>[2x]GSHMMPQLQFKDAFWCRDFTAHTGYEVLLQRLLDGRKMCKDMEELLRQRAQAEERYGKELVQIARKAGGQTEINSLRASFDSLKQQMENVGSSHIQLALTL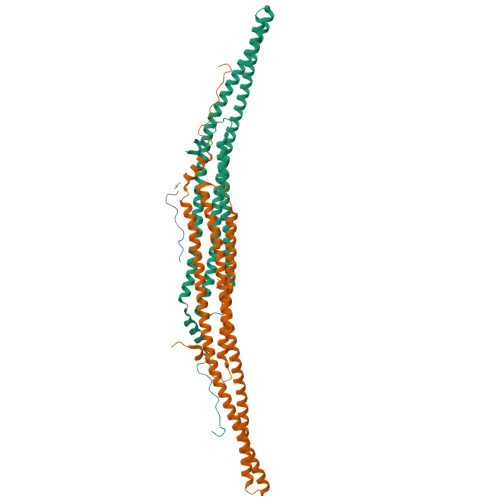REELRSLEEFRERQKEQRKKYEAVMDRVQKSKLSLYKKAMESKKTYEQKCRDADDAEQAFERISANGHQKQVEKSQNKARQCKDSATEAERVYRQSIAQLEKVRAEWEQEHRTTCEAFQLQEFDRLTILRNALWVHSNQLSMQCVKDDELYEEVRLTLEGCSIDADIDSFIQAKSTGTEPPAPVPYQNYYD;> GFANRFSKPKGPRNPPPTWNI> VKDTYTDRLDDWNGIIAGNQYYDSKNDQMAKLNQELEGKVADSLSSISSQADRIYLWEKFSNYKTSANLTATYRKLEEMAKQVTNPSSRYYQDETVVRTVRDSMEWMHKHVYNSEKSIVGNWWDYEIGTPRAINNTLSLMKEYFSDEEIKKYTDVIEKFVPDPEHFRKTTDNPVKALGGNLVDMGRVKVIAGLLRKDDQEISSTIRSIEQVFKLVDQGEGFYQDGSYIDHTNVAYTGAYGNVLIDGLSQLLPVIQKTKNPIDKDKMQTMYHWIDKSFAPLLVNGELMDMSRGRSISRANSEGHVAAVEVLRGIHRIADMSEGETKQRLQSLVKTIVQSDSYYDVFKNLKTYKDISLMQSLLSDAGVASVPRTSYLSAFNKMDKTAMYN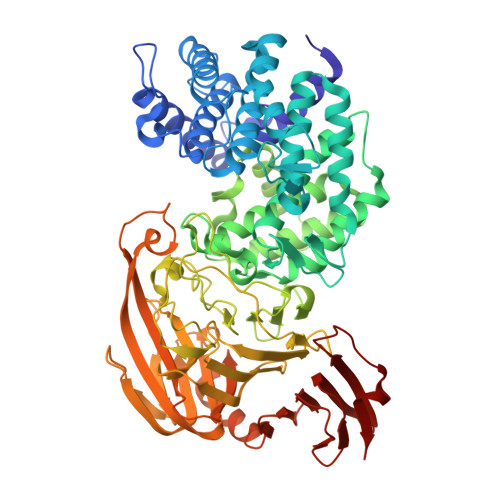AEKGFGFGLSLFSSRTLNYEHMNKENKRGWYTSDGMFYLYNGDLSHYSDGYWPTVNPYKMPGTTETDAKRADSDTGKVLPSAFVGTSKLDDANATATMDFTNWNQTLTAHKSWFMLKDKIAFLGSNIQNTSTDTAATTIDQRKLESSNPYKVYVNDKEASLTEQEKDYPETQSVFLESSDSKKNIGYFFFKKSSISMSKALQKGAWKDINEGQSDKEVENEFLTISQAHKQNGDSYGYMLIPNVDRATFNQMIKELESSLIENNETLQSVYDAKQGVWGIVKYDDSVSTISNQFQVLKRGVYTIRKEGDEYKIAYYNPETQESAPDQEVFKKL>STEAQEGVIKVATQSETVTGTSANTAVSPKNLKWIAQSEPTWAATTAIRGFVKTSSGSITFVGNDTVGSTQDLELYEKNSYAVSPYELNRVLANYLPLKAKAADTNLLDGLDSSQFIRRDIAQTVNGSLTLTQQTNLSAPLVSSSTGEFGGSLAANRTFTIRNTGAPTSI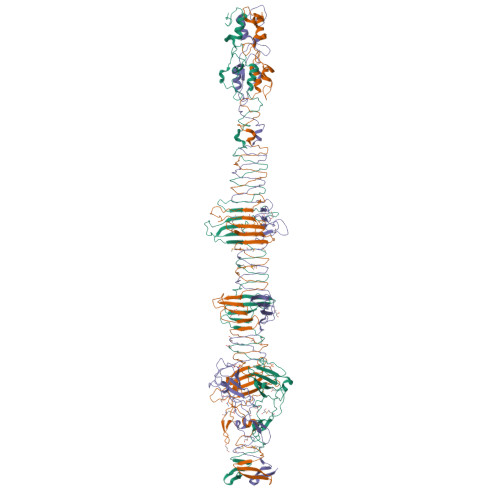VFEKGPASGANPAQSMSIRVWGNQFGGGSDTTRSTVFEVGDDTSHHFYSQRNKDGNIAFNINGTVMPININASGLMNVNGTATFGRSVTANGEFISKSANAFRAINGDYGFFIRNDASNTYFLLTAAGDQTGGFNGLRPLLINNQSGQITIGEGLIIAKGVTINSGGLTVNSRIRSQGTKTSDLYTRAPTSDTVGFWSIDINDSATYNQFPGYFKMVEKTNEVTGLPYLERGEEVKSPGTLTQFGNTLDSLYQDWITYPTTPEARTTRWTRTWQKTKNSWSSFVQVFDGGNPPQPSDIGALPSDNATMGNLTIRDFLRIGNVRIVPDPVNKTVKFEWVE[3x]>[2x]HMDTTFQAAIDTGKINGAVVCATDAQGHFVYNKATGERTLLSGEKQPQ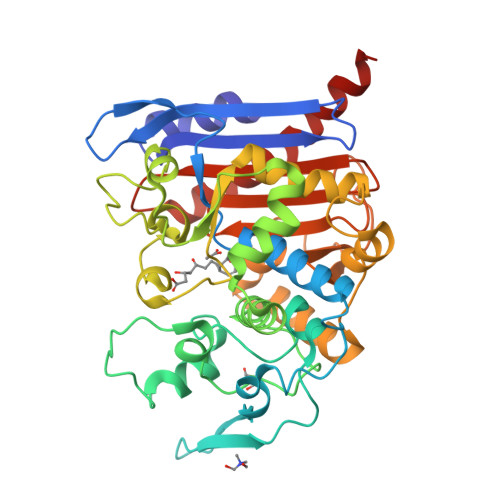QLDDVLYLASATKLITTIAALQCVEDGLLSLDGDLSSIAPELAAKYVLTGFTDDESPLDDPPARPITLKMLLTHSSGTSYHFLDPSIAKWRAQYANPENEKPRLVEEMFTYPLSFQPGTGWMYGPGLDWAGRVVERVTGGTLMEFMQKRIFDPLGITDSQFYPVTREDLRARLVDLNPSDPGALGSAVIGGGGEMNLRGRGAFGGHGLFLTGLDFVKILRSLLANDGMLLKPAAVDNMFQQHLGPEAAASHRAALASPLGPFFRVGTDPETKVGYGLGGLLTLEDVDGWYGERTLTWGGGLTLTWFIDRKNNLCGVGAIQAVLPVDGDLMADLKQTFRHDIYRKYSAWKGQQ> CCAIDQDFLDAAGILENEAIDIWNVTNGKRFSTYAIAAERGSRIISVNGAAAHCASVGDIVIIASFVTMPDEEARTWRPN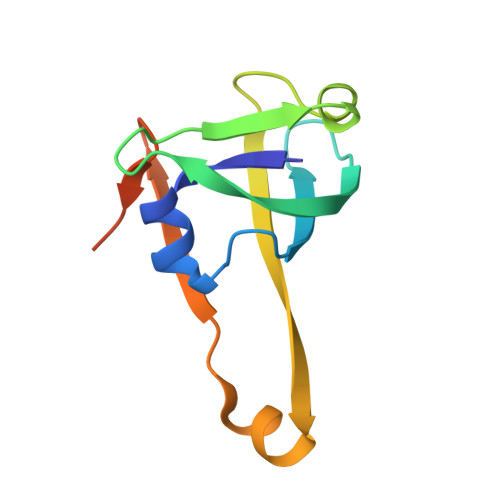VAYFEGDNEMKRTAKAIPVQVA>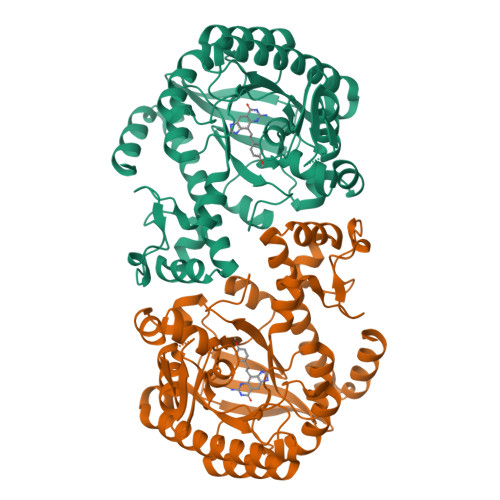[2x]VEATAQETDRPRFSFSIAAREGKARTGTIEMKRGVIRTPAFMPVGTAATVKALKPETVRATGADIILGNTYHLMLRPGAERIAKLGGLHSFMGWDRPILTDSGGYQVMSLSSLTKQSEEGVTFKSHLDGSRHMLSPERSIEIQHLLGSDIVMAFDECTPYPATPSRAASSMERSMRWAKRSRDAFDSRKEQAENAALFGIQQGSVFENLRQQSADALAEIGFDGYAVGGLAVGEGQDEMFRVLDFSVPMLPDDKPHYLMGVGKPDDIVGAVERGIDMFDCVLPTRSGRNGQAFTWDGPINIRNARFSEDLKPLDSECHCAVCQKWSRAYIHHLIRAGEILGAMLMTEHNIAFYQQLMQKIRDSISEGRFSQFAQDFRARYFARNS> MFQQLSARLQEAIGRLRGRGRITEEDLKATLREIRRALMDADVNLEVARDFVERVREEALGKQVLESLTPAEVILATVYEALKEALGGEARLPVLKDRNLWFLVGLQGSGKTTTAAKLALYYKGKGRRPLLVAADTQRPAAREQLRLLGEKVGVPVLEVMDGESPESIRRRVEEKARLEARDLILVDTAGRLQIDEPLMGELARLKEVLGPDEVLLVLDAMTGQEALSVARAFDEKVGVTGLVLT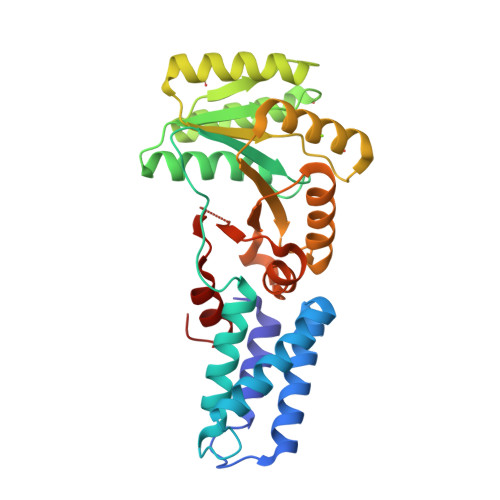KLDGDARGGAALSARHVTGKPIYFAGVSEKPEGLEPFYPERLAGRILGMG>[4x]MGSDKIHHHHHHMPKVTVSIKVVPAVEDGRLHEVIDRAIEKISS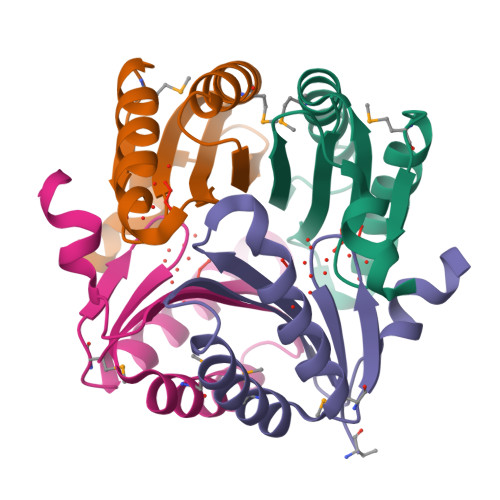WGMKYEVGPSNTTVEGEFEEIMDRVKELARYLEQFAKRFVLQLDIDYKAGGITIEEKVSKYR>[2x]MRGSHHHHHHGSMIFDKEDYKAFDPELWNAIDAEAERQQNNIELIASENVVSKAVMAAQGTLLTNKYAE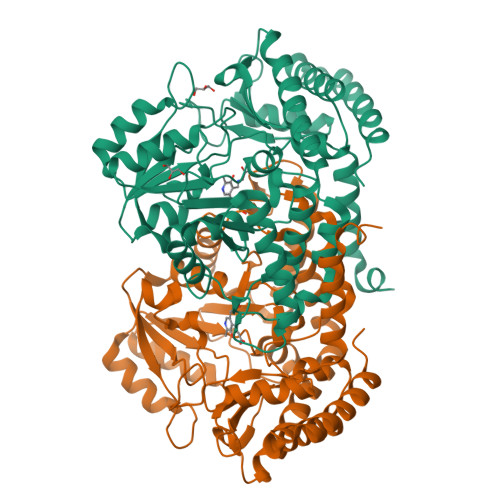GYPGKRYYGGTAVIDVVETLAIERAKKLFGAKFANVQPHSGSQANAAVYMSLIQPGDTVMGMDLSAGGHLTHGAPVSFSGKTYNFVSYNVDKESELLDYDAILAQAKEVRPKLIVAGASAYSRIIDFAKFREIADAVGAYLMVDMAHIAGLVASGHHPSPVPYAHVTTTTTHKTLRGPRGGLILTDDEDIAKKLNSAVFPGLQGGPLEHVIAAKAVALKEALDPAFKEYGENVIKNAAAMADVFNQHPDFRVISGGTNNHLFLVDVTKVVENGKVAQNVLEEVNITLNKNSIPYEQLSPFKTSGIRVGSPAITSRGMGEAESRQIAEWMVEALENHDKPEVLERIRGDVKVLTDAFPLY>[4x]TTIVSVRRNGHVVIAGDGQATLGNTVMKGNVKKVRRLYNDKVIAGFAGGTADAFTLFELFERKLEMHQGHLVKAAVELAKDWRTDRMLRKLEALLAVADETASLIITGNGDVVQPENDLIAIGSGGPYAQAAARALLENTELSAREIAEKALDIAGDICIYTNHFHTIEELSYKA;>[2x]HHHHHHHSEMTPREIVSELDKHIIGQDNAKRSVAIALRNRWRRMQLNEELRHEVTPKNILMIGPTGVGKTEIARRLAKLANAPFIKVEATKFTEVGYVGKEVDSIIRDLTDAAVKMVRVQAIEKNRYRAEELAEERILDVLIPPAKNNWGQTEQQQEPSAARQAFRKKLREGQLDDKEIEIDLAAAPMGVE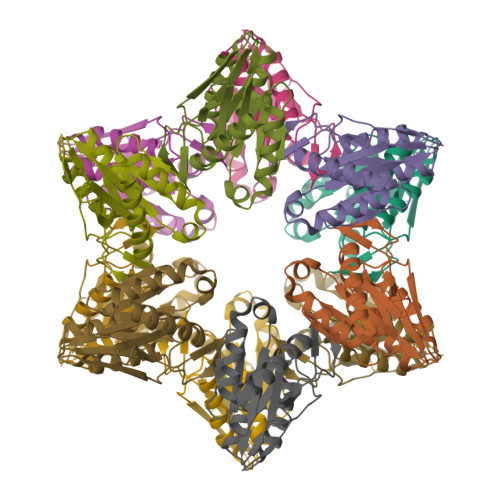IMAPPGMEEMTSQLQSMFQNLGGQKQKARKLKIKDAMKLLIEEEAAKLVNPEELKQDAIDAVEQHGIVFIDEIDKICKRGESSGPDVSREGVQRDLLPLVEGCTVSTKHGMVKTDHILFIASGAFQIAKPSDLIPELQGRLPIRVELQALTTSDFERILTEPNASITVQYKALMATEGVNIEFTDSGIKRIAEAAWQVNESTENIGARRLHTVLERLMEEISYDASDLSGQNITIDADYVSKHLDALVADEDLSRFIL> ETHRRVRLLKHGSDKPLGFYIRDGTSVRVTASGLEKQPGIFISRLVPGGLAESTGLLAVNDEVIEVNGIEVAGKTLDQVTDMMVANSSNL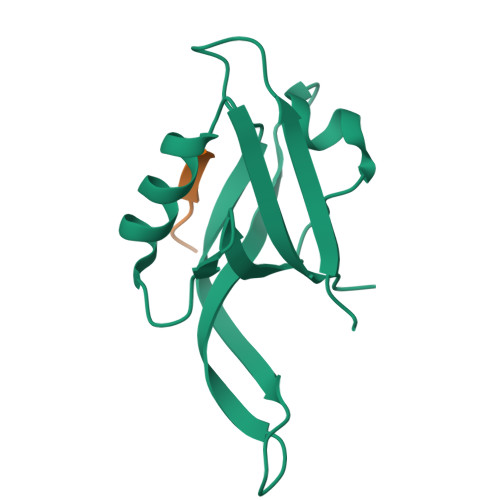IITVKPAN;> XVKESLV[5-(aminomethyl)-6-(2,2-dimethylpropyl)-2-ethyl-4-(4-methylphenyl)pyridin-3-yl]acetic acid | 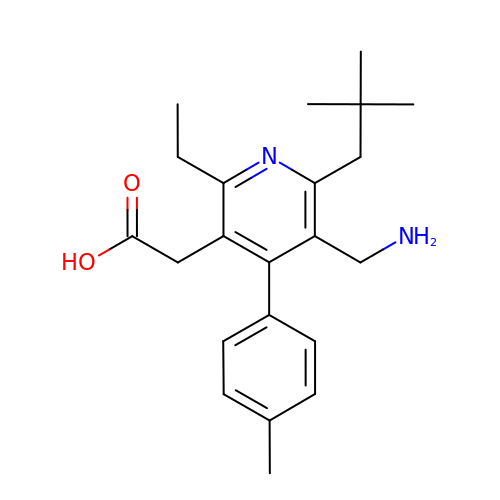C22 H30 N2 O2 | HQVOROHHYWZJLD-UHFFFAOYSA-N8-(3-(3-aminobenzamido)-4-methylbenzamido)naphthalene-1,3,5-trisulfonic acid | C25 H21 N3 O11 S3 | 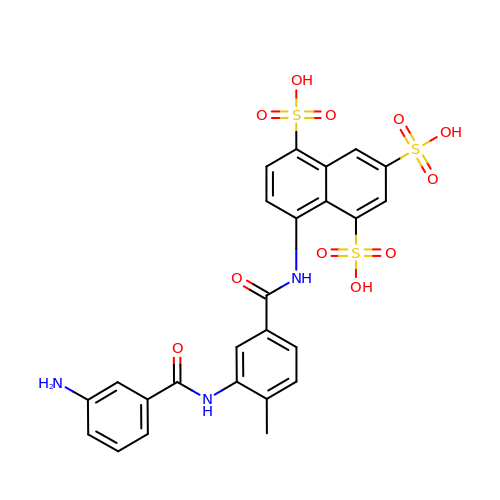FWPDBHFZCRXISJ-UHFFFAOYSA-N>[2x]M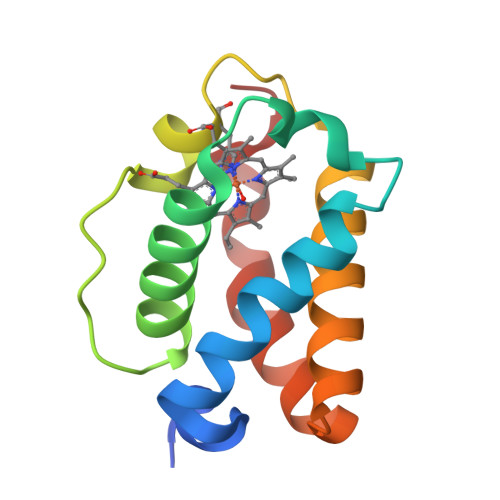NKPQTIYEKLGGENAMKAAVPLFYKKVLADERVKHFFKNTDMDHQTKQETDFLTMLLGGPNHYKGKNMTEAHKGMNLQNLHFDAIIENLAATLKELGVTDAVINEAAKVIEHTRKDMLGK1-[5-(4-amino-2,7-dimethyl-7H-pyrrolo[2,3-d]pyrimidin-5-yl)-2,3-dihydro-1H-indol-1-yl]-2-[3-fluoro-5-(trifluoromethyl)phenyl]ethanone 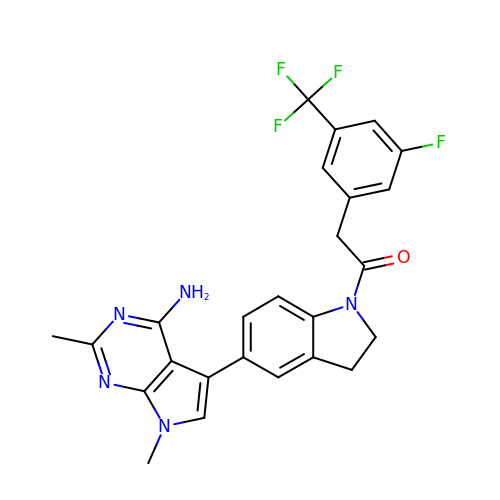| C25 H21 F4 N5 O | MXBMIZHUPORZGB-UHFFFAOYSA-N> AKKYAVVLKTLTDPFWQSMKAGIEAEAKELGVTVDIFAAASEGDAEAQLALFESLSNKNYKGIAFAPLTADNLVEPVASAWKKGTYLVNLDDKIDMKALKAAGGNVEAFVTTDNVAVGAQGAGYIIEKLGAEGGEVAIIEGEAGNAAGEARTKGATDAFDKASNIKLVASQPADWDRAKAKQVATDILAKHPNIKAIYCANDTMALGVAQAVADAGKTGKVLVVGTDGIPEAQQAVKAGKMTATV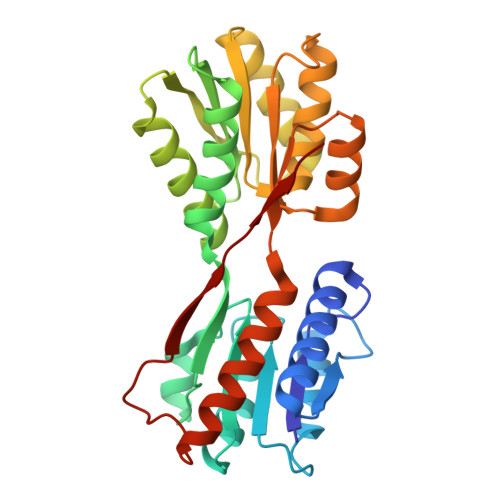AQNPAAIGATGLKLMVDAQKKGKVIPLDKKPQYVLVASKLVTK5'-deoxy-5'-[({6-[(alpha-D-galactopyranosyloxy)methyl]pyridin-2-yl}carbonyl)amino]uridine 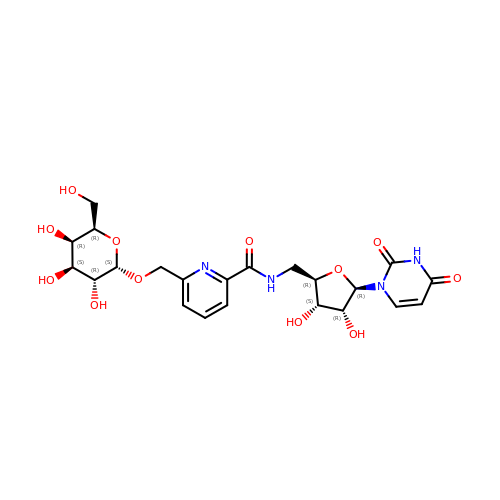| C22 H28 N4 O12 | KPOTWZYLDCHCIG-DSVOXYOZSA-N> HHHHHHSSGLVPRGSHMVRDGNGTSRRDVFEVFSRDGTPIRGFSRPGPGETVVLVHGVAMDRRIWAESGFLDALPDAHVLALDLRGRGESGRVGTAEGHALRRYVEDVRAVLDRFGRARYSLFGTFFGGRIALQVA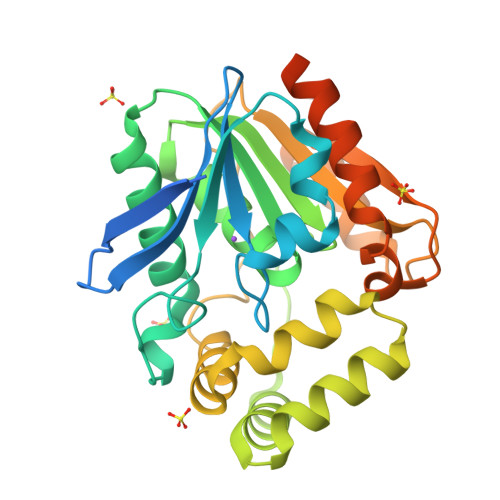AVDTRVARAFSFCAHAEQVEIPEDAVEEEAVAVEGPGGHAYLRDHFTGRGAPPWMVEACARVDPGELGAATRGLLHGSDRRTERGHPDQELVLITADGDADLAPFHAGERRLGAHLWLVDAPTRIKAAGRLAEVGRRVAGVLAEGGHGTGDAPAEARTTGDAPAEARASGTGVV>NKEVIPPENFSHVVGEIYRSSFPRQENFSFLHERLKLKSILVLIPEEYPQENLNFLKLTGIKLYQVGMSGNKEPFVNIPSHLLTKAL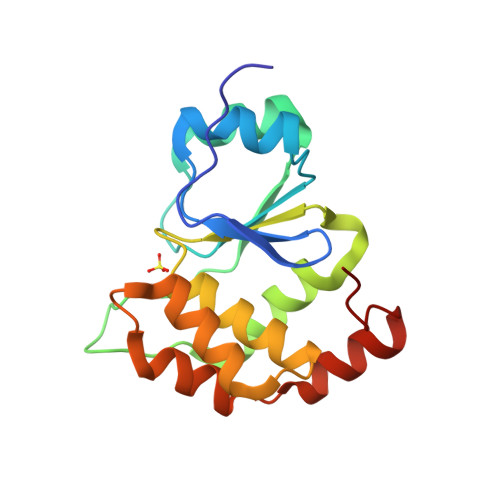EIVLNPANQPILIHSNRGKHRTGCLIGCIRKLQNWSLTMIFDEYRRFAFPKARALDQQFIEMYDDDEIKRIASKNNWLPLQW[24x]>[2x]MKKIEVYAQPDCPPCVIVKEFLKHNNVAYEEFDVKKDAAARNRLLYDYDSYSTPTVVIDGEVVAGFQIEKLQQLLNIE

Thioredoxin (Trx) and glutaredoxin (Grx) are small ubiquitous proteins acting as cysteine disulfide oxidoreductases in the cell and belong to the thioredoxin superfamily. The thioredoxin BC3987 found in B. cereus ATCC 14579 is conserved among all the members of the B. cereus group, including B. anthracis, B. mycoides, B. pseudomycoides, B. thuringiensis and B. weihenstephanensis. Like E. coli and C. ammoniagenes NrdH the BC3987 have a α/β/α Trx fold typical for all members of the Thioredoxin superfamily. The BC3987 protein has a C-P-P-C active site motif that differs from what is typically observed for Trxs and Grxs.

Substituting the conserved Thr8 that is close to the active site with Ala has altered the hydrogen bond network and the effect of this has been characterized. The BC3987 wild type and T8A mutant structures were refined to 1.4 and 1.18 Å, respectively. In the T8A mutant structure, all residues 1–78 are visible in the electron density map of the corresponding high quality chain. In the other chain, residues 3–76 are observed, with lacking density at the side chain atoms of Asn76. The crystal structure of the T8A mutant resembles the wild type structure and the C-P-P-C motifs in these structures superimpose with a RMSD value of 0.053. One possible explanation for this observation is that both cysteines in the reduced C-P-P-C active site have lowered pKa values. The pH-titration curves for wild type and T8A BC3987 in Figure 1 are similar in the pH interval 6.5–9, indicating that the nucleophilic Cys12 pKa value is not affected by the T8A mutation. Following the reasoning above, the wild type BC3987 has two titratable thiolates with pKa values 5.1 and 7.2 while the T8A mutant has one thiolate with a pKa value of 7.2 and a second thiolate that behave different from the wild type. The control reaction with insulin and DTT is very slow compared to the wild type and T8A mutant BC3987 catalyzed reactions. The efficiency of thioredoxin insulin reduction is measured in this assay, and from the curves in Figure 2 it can be concluded that the wild type BC3987 has a different reactivity towards the substrate compared to the T8A mutant. The lag-time before any precipitated insulin is observed is much longer for the T8A mutant, and the slope of the curve after the lag-period is slightly steeper for the wild type enzyme. Disturbing the hydrogen bonding networks by removing a highly conserved Thr residue near the buried Cys resulted in decreased efficiency for the BC3987 thioredoxin.>KANRQREPGLGFSFEFTEQQKEFQATARKFAREEIIPVAAEYDKTGEYPVPLIRRAWELGLMNTHIPENCGGLGLGTFDACLISEELAYGCTGVQTAIEGNSLGQMPIIIAGNDQQKKKYLGRMTEEPLMCAYCVTEPGAGSDVAGIKTKAEKKGDEYIINGQKMWITNGGKANWYFLLARSDPDPKAPANKAFTGFIVEADTPGIQIGRKELNMGQRCSDTRGIVFEDVKVPKENVLIGDGAGFKVAMGAFDKERPVVAAGAVGLAQRALDEATKYALERKTFGKLLVEHQAISFMLAEMAMKVELARMSYQRAAWEVDSGRRNTY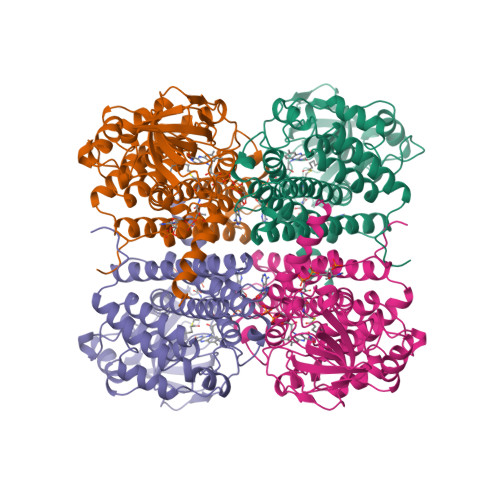YASIAKAFAGDIANQLATDAVQILGGNGFNTEYPVEKLMRDAKIYQIYGGTSQIQRLIVAREHIDKYKN[4x]>[2x]QQDWLTFQKKHITNTRDVDCDNIMSTNLFHCKDKNT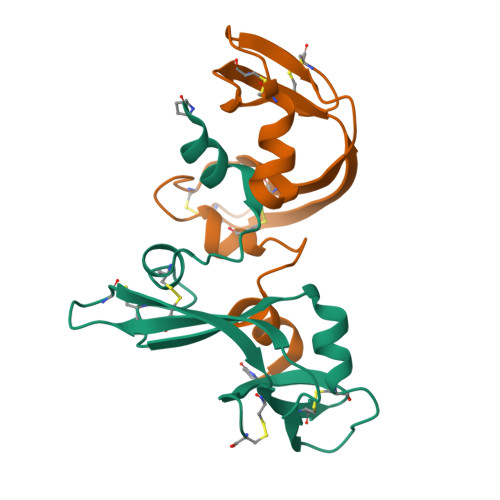FIYSRPEPVKAICKGIIASKNVLTTSEFYLSDCNVTSRPCKYKLKKSTNKFCVTCENQAPVHFVGVGSC Bone morphogenetic proteins (BMPs) are dimeric transforming growth factor β (TGFβ) family cytokines, initiating cellular signalling by forming a complex with two copies of type I receptors and two copies of type II receptors, both of which are type I transmembrane proteins with an intracellular serine/threonine kinase domain. Activin receptor-like kinase 1 (ALK1) is a type I receptor specifically expressed on endothelial cells, mediating the signals from BMP9 and BMP10 exclusively. ALK1-mediated endothelial BMP9 and BMP10 signalling plays many important roles in angiogenesis and the maintenance of vascular quiescence. All TGFβ family ligands are synthesised as preproproteins, processed by furin-like proprotein convertase upon secretion. It has been shown for several family members, including TGFβ, BMP9 and BMP10, that the prodomain remains tightly bound to the growth factor (GF) domain in circulation.

As expected, the ALK1 ECD binds BMP10 in a 2:2 stoichiometry, and the two ALK1 ECD monomers are not in direct contact. Using the PDBePISA server, a total of 26 BMP10 residues were identified at the ALK1 binding interface (lines over the sequence). Secondly, by solving the crystal structure of the BMP10:ALK1 complex and comparing it to published structures, we have identified three regions that are highly conserved between BMP9 and BMP10. The conserved region 1 accounts for ALK1 specificity. The most striking feature in the conserved region 2 is the insertion of a hydrophobic residue, Y416 in BMP9 and F411 in BMP10 (red arrow), located in the top strand of finger 1 (red arrows). This additional residue leads to a kink in this β-strand of BMP9 and BMP10, resulting in a novel conformation that allows BMP9 and BMP10 to form unique interactions.

> GDPVKPSRGPLVTCTCESPHCKGPTCRGAWCTVVLVREEGRHPQEHRGCGNLHRELCRGRPTEFVNHYCCDSHLCNHNVSLVLEATQPPSEQPGTDGQ;> NAKGNYCKRTPLYIDFKEIGWDSWIIAPPGYEAYECRGVCNYPLAEHLTPTKHAIIQALVHLKNSQKASKACCVPTKLEPISILYLDKGVVTYKFKYEGMAVSECGCR>[2x]GSHMSNTQTVLPFTGLNTPSGVAVDSAGTVYVTDHGNNRVVKLAA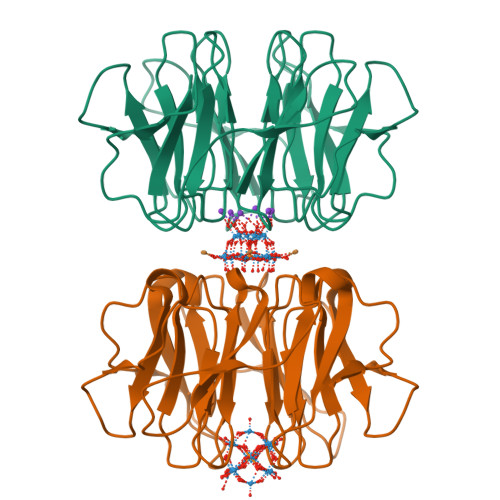GSNTQTVLPFTGLNTPSGVAVDSAGTVYVTDHGNNRVVKLAAGSNTQTVLPFTGLNTPSGVAVDSAGTVYVTDHGNNRVVKLAAGSNTQTVLPFTGLNTPSGVAVDSAGTVYVTDHGNNRVVKLAAGSNTQTVLPFTGLNTPSGVAVDSAGTVYVTDHGNNRVVKLAAGSNTQTVLPFTGLNTPSGVAVDSAGTVYVTDHGNNRVVKLAAG>MSGFKFLFFSPDGTLYGV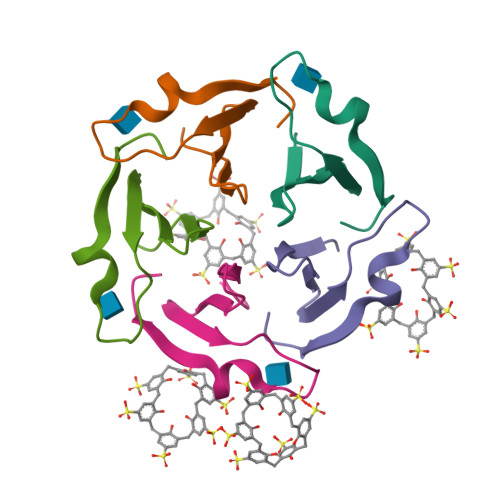HNDKLYKGTPPTSDKDNWLARATLIGNGGW[5x]> MSDDKIIRMANQIAAFFAVQPGDRAGPVAAHISE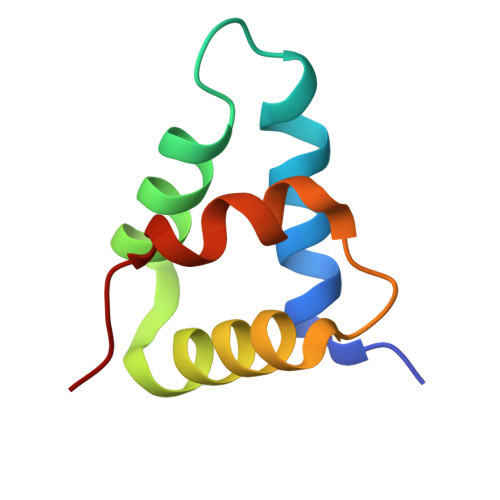NWSAPMRAALLAHVAAQSPGLDPLVIAAAPQIRPVPA>[2x]MVQYIFTPWRNRAELLAVRAQFYPEHTSKTHLKKHHQSTFQDDEHIRSEKQKAVARVSMWMQRGGCPHMVESTALLVAAILSDEAQGSGAAGGYAVRAAYSAAFSRFVTGLLDSHQDKQRKQSMYDVAKAVGLPAAFVELRHQATHEQLPSLTRLRSAARRALEWIWWYYWKGLGPVDMVQRGVNGKGVAGVGDTSESEEKDVGEEGGDAAARCREGVVRLLESDVRVGGEAINGPGKEELLAEFGEALVLTTLDAAAGNTRDVGVLRRAIGLMREIVNGGDEDCMQLENGKGNRDVEKLKEELKKGWEEIKRLAQEKEDSGDDQTEDEDVDMEAEEEDKKEQQSGWVLYDEKEWVPKPIGIV;>MTSTKKRKLEGSASESGNNTPILSAFAARQQLWAQSLVVQAQKQPQSVDNSKHVTERRSATPI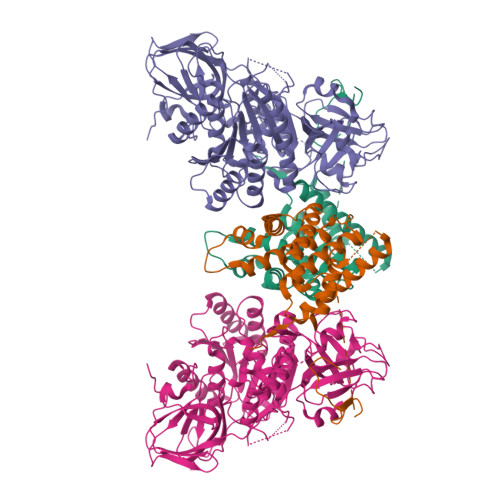SAAQVLRKSKRKSPEDSPITPATPATPVETEEEKPSKPSSPRELLRHHSSFQPNNSNFQRKAGGRLVLSTPDVERFVILGNYGVKVHQGEVTIAGATLTPIDDVQWVHAPHCHALPVLRTANDTVIELLPCPTAQGLRELARLNPLFGRLWNETSDTFQIIYTSADAPKRTSLRELASHPAWNKKISELLTSTRRKPSPILFICGPKSSGKSTFGRLLTNRLMTDRAGHKSRSWKPVMVLDLDPGQPEFSPPGVVSLTKLRRPNLAPPFCHPGLSFGEKGLDGGNEGMTTVRMHAIASVTPALDPAHFIACARDLFAYYRRSASQENIPLVVNTPGWIQGTGLDLLAELIAVLRPTEVLYMSEDGPEETVSALREACASSSTIPFTMLPSQPNSSGEGGGGGAASWTPATLRSMAMQSYFHLSPFSRDQQGGPGCEWNPTPLTHLCPWRVRLAGRPDERGVLGIVCYDHQYAPELVSDAINGMVMGLVRIEKKEALRGLAVPGDTSLSFTSSTSQGGCDDELDSDSNSSSAPSFTSSSPSHLNSTPLLPLIPNPTGSPLSPQYTSLVGLVLIRGVSLTASNPELHLLTPVPPSVLHSFRGDELVLVAGKFDAPTWAYVEGLYWKSNSKAAKRVDEEREDEDREESGGVEEEEEQDEVPWVEMLHGSAGRDVGSRVWRVRRDLGRS[2x]> MGSSHHHHHHSQDPMDYFNIKQNYYTGNFVQCLQEIEKFSKVTDNTLLFYKAKTLLALGQYQSQDPTSKLGKVLDLYVQFLDTKNIEELENLLKDKQNSPYELYLLATAQAILGDLDKSLETCVEGIDNDEAEGTTELLLLAIEVALLNNNVSTASTIFDNYTNAIEDTVSGDNEMILN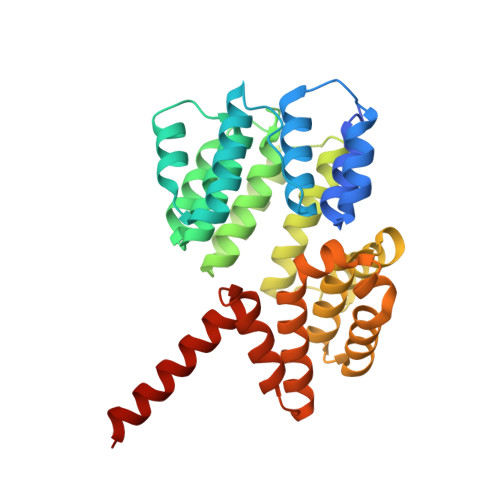LAESYIKFATNKETATSNFYYYEELSQTFPTWKTQLGLLNLHLQQRNIAEAQGIVELLLSDYYSVEQKENAVLYKPTFLANQITLALMQGLDTEDLTNQLVKLDHEHAFIKHHQEIDAKFDELVRKYDTSN> GHHHHHHGSGSGENLYFQGGGSGVSLGQALLILSVAALLGTTVEEAVKRALWLKTK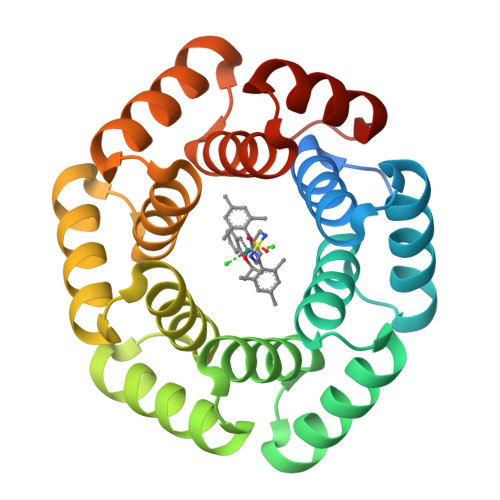LGVSLEQAARTLSVAAYLGTTVEEAVKRALKLKTKLGVSLEQALLILFAAAALGTTVEEAVKRALKLKTKLGVSLEQALLILWTAVELGTTVEEAVKRALKLKTKLGVSLGQAQAILVVAAELGTTVEEAVYRALKLKTKLGVSLGQALLILEVAAKLGTTVEEAVKRALKLTTKLG2-[(3-bromobenzene-1-carbonyl)amino]-6-{[(4-carboxy-5-methylfuran-2-yl)sulfonyl]amino}-2,6-dideoxy-alpha-D-glucopyranos e | C19 H21 Br N2 O10 S | 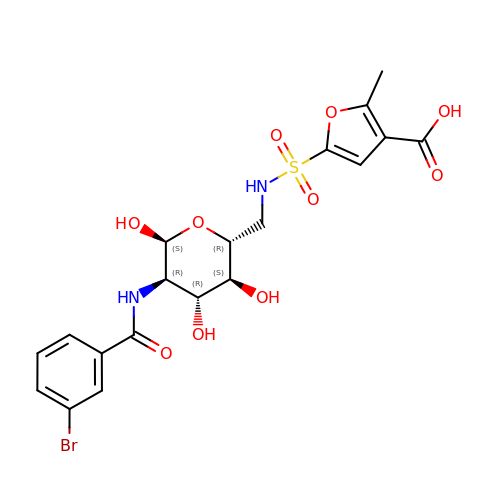GEVMYBPXLUPCSS-OREGDWJXSA-N>SLVC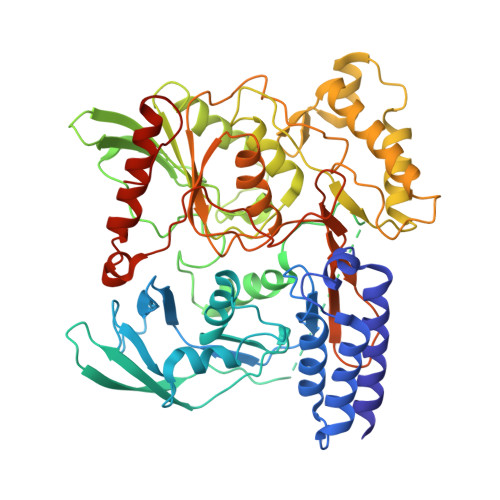KNALQDLSFLEHLLQVKYAPKTWKEQYLGWDLVQSSVSAQQKLRTQENPSTSFCQQVLADFIGGLNDFHAGVTFFAIESAYLPYTVQKSSDGRFYFVDIMTFSSEIRVGDELLEVDGAPVQDVLATLYGSNHKGTAAEESAALRTLFSRMASLGHKVPSGRTTLKIRRPFGTTREVRVKWRYVPEGVGDLATIAPSIRAPQLQKSMRSFFPKKDDAFHRSSSLFYSPMVPHFWAELRNHYATSGLKSGYNIGSTDGFLPVIGPVIWESEGLFRAYISSVTDGDGKSHKVGFLRIPTYSWQDMEDFDPSGPPPWEEFAKIIQVFSSNTEALIIDQTNNPGGSVLYLYALLSMLTDRPLELPKHRMILTQDEVVDALDWLTLLENVDTNVESRLALGDNMEGYTVDLQVAEYLKSFGRQVLNCWSKGDIELSTPIPLFGFEKIHPHPRVQYSKPICVLINEQDFACADFFPVVLKDNDRALIVGTRTAGAGGFVFNVQFPNRTGIKTCSLTGSLAVREHGAFIENIGVEPHIDLPFTANDIRYKGYSEYLDKVKKLVCQLINNDGTIILAEDGSFHHHHHH[2x]> APLAPASYHPKPWLGAQPATVVTPGVNVTLRCRAPQPAWRFGLFKPGEIAPLLFRDVSSELAEFFLEEVTPAQGGSYRCCYRRPDWGPGVWSQPSDVLELLVTEELPRPSLVALPGPVVGPGANVSLRCAGRLRNMSFVLYREGVAAPLQYRHSAQPWADFTLLGARAPGTYSCYYHTPSAPYVLSQRSEVLVIAA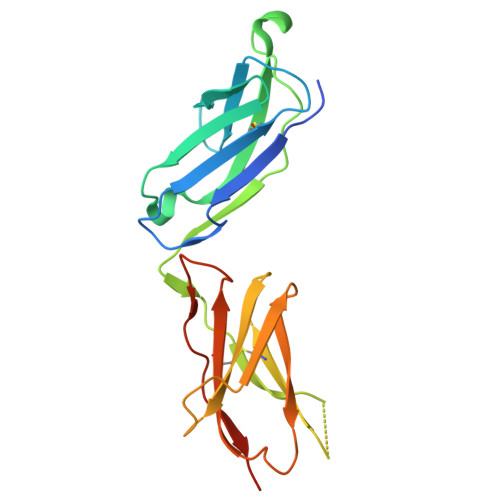AHHHHHH> QSCATGPRNCKDLLDRGHFLSGWHTIYLPDCRPLTVLCDMDTDGGGWTVFQRRMDGSVDFYRDWAAYKQGFGSQLGEFWLGNDNIHALTAQGSSELRTDLVDFEGNHQFAKYKSFKVADEAEKYKLVLGAFVGGSAGNSLTGHNNNFFSTKDQDNDVSSSNCAEKFQGAWWYADCHASNLNGLYLMGPHESYANGINWSA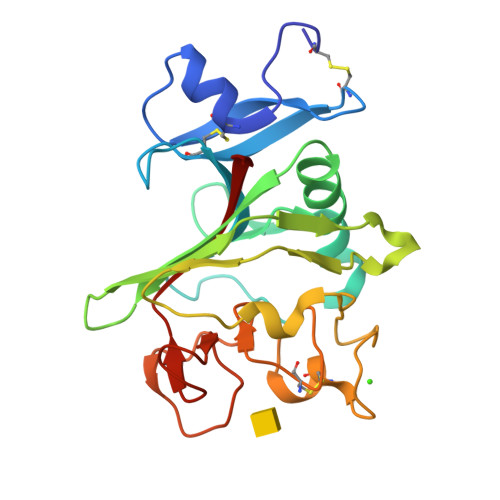AKGYKYSYKVSEMKVRPA>MSLTITPLSPALGAQISGVDISRDISAEERDAIEQALLQHQVLFLRDQPINPEQQARFAARFGDLHIHPIYPNVPDTPQVLVL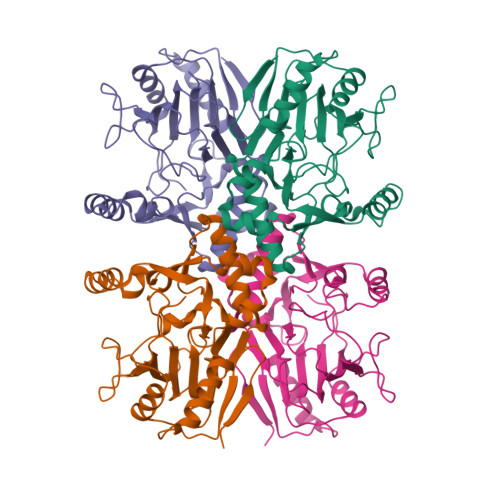DTAVTDVRDNAVWHTDVTFLPTPALGAVLSAKQLPAYGGDTLWASGIAAFEALSAPLREMLDGLTATHDFTKSFPLERFGTTPQDLARWEATRRNNPPLSHPVVRTHPVSGRKALFVNEGFTTRINELSELESDALLRLLFAHATRPEFSIRWRWQENDVAFWDNRVTQHFAVDDYRPNRRVMHRATILGDAPF[4x]GEMCITABINE DIPHOSPHATE | C9 H13 F2 N3 O10 P2 | 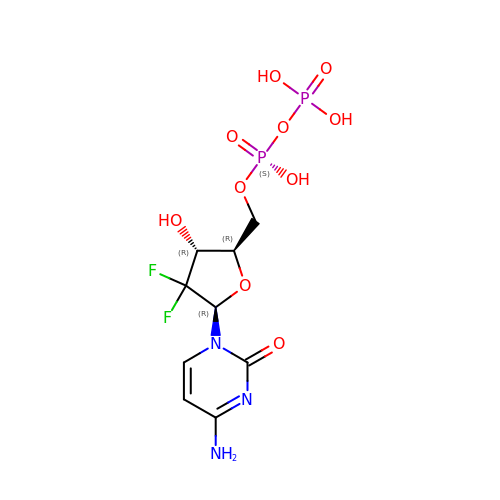FRQISCZGNNXEMD-QPPQHZFASA-N(14S,17R)-20-amino-17-hydroxy-11,17-dioxo-12,16,18-trioxa-17lambda~5~-phosphaicosan-14-yl 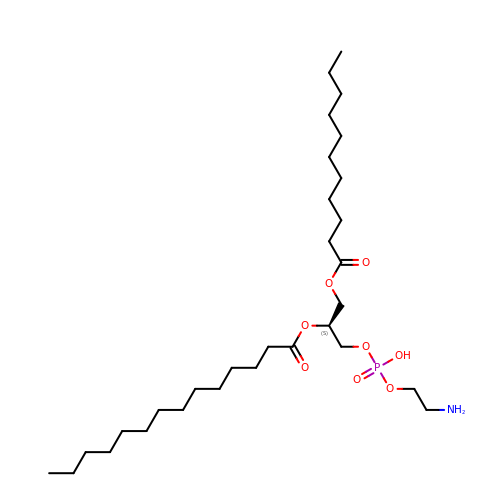tetradecanoate | C30 H60 N O8 P | BMOFTHAXXFOIRF-NDEPHWFRSA-N> GPGSCPTHADSLNNLANIKREQGNIEEAVRLYRKALEVFPEFAAAHSNLASVLQQQGKLQEALMHYKEAIRISPTFADAYSNMGNTLKEMQDVQGALQCYTRAIQINPAFADAHSNLASIHKDSGNIPEAIASYRTALKLKPDFPDAYCNLAHCLQIVCDWTDYDERMKKLVSIVADQLEKNRLPSVHPHHSMLYPLSHGFRKAIAERHGNLCLDKINVLHKPPYEHPKDLKLSDGRLRVGYVSSDFGNHPTSHLMQSIPGMHNPDKFEVFCYALSPDDGTNFRVKVMAEANHFIDLSQIPCNGKAADRIHQDGIHILVNMNGYTKGARNELFALRPAPIQAMWLGYPGTSGALFMDYIITDQETSPAEVAEQYSEKLAYMPHTFFIGDHANMFPHLKKKAVIDFKSNGHIYDNRIVLNGIDLKAFLDSLPDVKIVKMKCPDGGDNADSSNTALNMPVIPMNTIAEAVIEMINRGQIQITINGFSISNGLATTQINNKAATGEEVPRTIIVTTRSQYGLPEDAIVYCNFNQLYKIDPSTLQMWANILKRVPNSVLWLLRFPAVGEPNIQQYAQNMGLPQNRIIFSPVAPKEEHVRRGQLADVCLDTPLCNGHTTGMDVLWAGTPMVTMPGETLASRVAASQLTCLGCLELIAKNRQEYEDIAVKLGTDLEYLKKVRGKVWKQRISSPLFNTKQYTMELERLYLQMWEHYAAGNK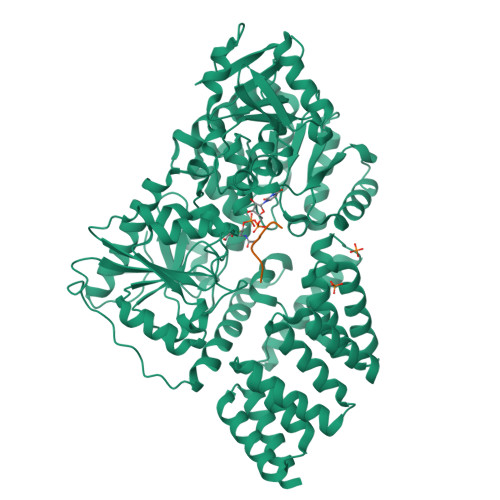PDHMIKPVE;> VTPVSTAA>MIFSVDKVRADFPVLSREVNGLPLAYLDSAASAQKPSQVIDAEAEFYRHGYAAVHRGIHTLSAQATEKMENVRKRASLFINARSAEELVFVRGTTEGINLVANSWGNSNVRAGDNIIISQMEHHANIVPWQMLCARVGAELRVIPLNPDGTLQLETLPTLFDEKTRLLAITHVSNVLGTENPLAEMITLAHQHGAKVLVDGAQAVMHHPVDVQALDCDFYVFSGHKLYGPTGIGILYVKEALLQEMPPWEGGGSMIATVSLSEGTTWTKAPWRFEAGTPNTGGIIGLGAALEYVSALGLNNIAEYEQNLMHYALSQLESVPDLTLYGPQNRLGVIAFNLGKHHAYDVGSFLDNYGIAVRTGHHCAMPLMAYYNVPAMCRASLAMYNTHEEVDRLVTGLQRI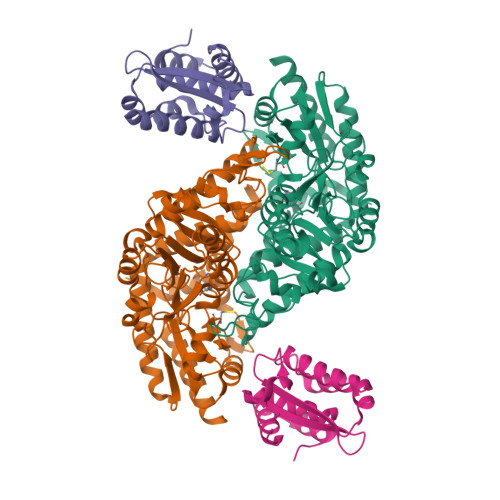HRLLG[2x];>MALLPDKEKLLRNFLRCANWEEKYLYIIELGQRLPELRDEDRSPQNSIQGAQSQVWIVMRQNAQGIIELQGDSDAAIVKGLIAVVFILYDQMTPQDIVNFDVRPWFCKMALTQHLTPSRSQGLEAMIRAIRAKAAALS[2x]>EAEAEFGACGAIASTVPNYNNAKLPDPFTFANGTALRTKADWSCRRAEISALIQNYEAGTLPPKPPVVTASFSKSGNTGTLAITAGLSNSQTIKFSPTISYPSGTPPANGWPLIIAYEGGSIPIPAGVATLTYSNSDMAQQNSASSRGQGLFYQLYGSTHSASAMTAWVWGVSRIIDALEMTPTAQINTQRIGVTGCARDGKGALMAGAFEERIALTIPQESGSGGDACWRLSKYEIDNGNQVQDAVEIVGENVWFSTNFNNYVQKLPTVPEDHHLLAAMVAPRAMISFENTDYLWLSPMSSFGCMTAAHTVWQGLGIADSHGFAQVGGHAHCAWPSSLTPQLNAFINRF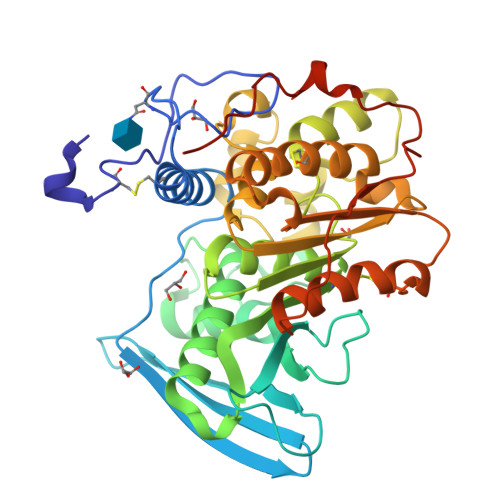LLDQSATTNVFTTNNQFGKVQWNAANWITWTTPTLTENLYFQGVDHHHHHH[2x]> ARIRAPQEATVKEVHDAPAVRGSIIANMLQEHDNPFTLYPYDTNYLIYTQTSDLNK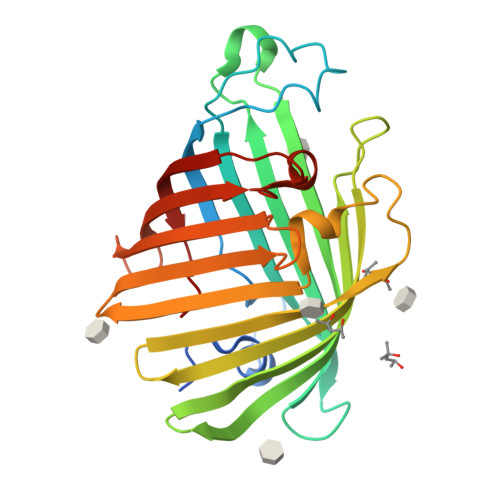EAIASYDWAENARKDEVKFQLSLAFPLWRGILGPNSVLGASYTQKSWWQLSNSEESSPFRETNYEPQLFLGFATDYRFAGWTLRDVEMGYNHDSNGRSDPTSRSWARLYTRLMAENGNWLVEVKPWYVVGNTDDNPDITKYMGYYQLKIGYHLGDAVLSAKGQYNWNTGYGGAELGLSYPITKHVRLYTQVYSGYGESLIDYNFNQTRVGVGVMLNDLF Escherichia coli NleB1, Citrobacter rodentium NleB, and Salmonella enterica SseK1/3 type III effectors fatally glycosyltransfer N-acetyl glucosamine (GlcNAc) from UDP-GlcNAc to arginine residues of death domain-containing proteins that regulate host inflammation, intra-bacterial proteins, and themselves, whose post-translational modification disrupts host immune functions and prolongs bacterial viability inside host cells. All NleB/SseK orthologs have a typical GT-A conformation with two abutting β/α/β Rossmann domains unlike a GT-B consisting of facing each other β/α/β Rossmann domains with a flexible linkage and share a high degree of structural similarity. Several structural cores were revealed for the new arginine N-glycosylation systems: a catalytic DxD motif to position the Mn2+ cofactor and UDP-GlcNAc donor substrate, His-Glu-Asn (HEN) motif to select UDP-GlcNAc as a suitable donor substrate before other sugar donors such as UDP-Glc/Gal, C-terminal loop to stably embrace the UDP-GlcNAc donor substrate, and Helix-Loop-Helix (HLH) domain predicted to select the acceptor targets. The SseK1 effector GlcNAcylates Arg9, Arg190, Arg160, and Arg149 of four proteins involved in methylglyoxal detoxification, namely, GloA, GloB, GloC, and YajL, respectively, and catalyze methylglyoxal detoxification to significantly enhance their activity.

All N-glycosylated NleB/SseKs form a Type-I-turn in the DxD motif in the ligand-bound state, and the pathogenic NleB1/SseK1/3 toxins also retain Type-I-turn in the DxD motif in the apo state. All solved N-glycosyltransferase NleB/SseKs structures were revisited to analyze the characteristic topology of the catalytic DxD motif and this analysis was extended to all structures of O-linked bacterial glycosylation toxins to determine whether these DxD motifs follow the characteristic topology. This revealed that in all ligand-bound N-/O-glycosylation toxins, the backbone of the DxD motif forms a Type I β-turn, in which the four residues (labeled i to i + 3) specifically form a pseudo-cycle C10 H-bond network between the backbone CO(i) and NH(i + 3) groups, and that the first aspartate binds with its next-but-one tyrosine, named as the YD bond, which allows the DxD motif to optimally bind Mn2+ and the donor substrates. In all apo- and UDP-bound NleB1/SseK1/SseK3 effectors, the DxD motifs lie in the 219YLDADM224/221YLDADM226/224YLDADM229 regions and their quaternary DADM motifs form a Type-I-turn by H-bonding between the backbone CO(i) and NH(i + 3) groups, while the free Asp oxygen (Oδ of Asp221/Asp223/Asp/226) in the DxD motif interacts with the hydroxyl oxygen (Oη of Tyr219/Tyr221/Tyr224), named as a YD bond.

> FTSFNGKDYPLCFLDEKTPLLFQWFERNPARFGKNDIPIINTEKNPYLNNIIKAATIEKERLIGIFVDGDFFPGQKDAFSKLEYDYENIKVIYRNDIDFSMYDKKLSEIYMENISKQESMPEEKRDCHLLQLLKKELSDIQEGNDSLIKSYLLDKGHGWFDFYRNMAMLKAGQLFLEADKVGCYDLSTNSGCIYLDADMIITEKLGGIYIPDGIAVHVERIDGRASMENGIIAVDRNNHPALLAGLEIMHTKFDADPYSDGVCNGIRKHFNYSLNEDYNSFCDFIEFKHDNIIMNTSQFTQSSWAR>MHHHHHHPNNFPAKLWRLVNS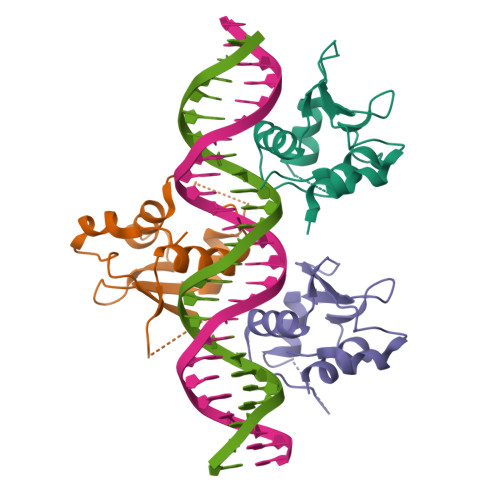PRYRSIRWDGRGEGLLIDQPLFEAELLSPPGPGGGGGTAGAGAEPELFKTTSFTSFIRQLNLYGFRKVVLGGPGGGKPAGNGPLHHFHNPHFRRDQPQLLVHLKRLTS[6x]The FAD synthetase from Corynebacterium ammoniagenes (CaFADS) is a bifunctional enzyme responsible for the synthesis of flavin mononucleotide (FMN) and flavin adenine dinucleotide (FAD) cofactors. The C-terminal module catalyzes FMN synthesis from riboflavin (RF) (riboflavin kinase, RFK), while the N-terminal one transforms FMN into FAD (FMN:adenylyltransferase, FMNAT). Bioinformatic tools for the exploration of macromolecular interfaces predict that CaFADS might stabilize in hexameric assemblies in solution, organized as dimer of trimers. In the predicted CaFADS dimer of trimers model, the protomers adopt a head-to-tail organization within each trimer that causes the RFK and FMNAT catalytic sites of two neighboring protomers 6 to be in proximity.

The overall structures of F206W, D298E and E301A CaFADSs are quite similar to that of the WT (A chains r.m.s.d. values 0.149, 0.152 and 0.251 Å, superimposing 274, 309 and 317 atoms, respectively). The E301A structure shows all residues in chain A but lacks 260, 261 and 262 in chain B. All mutant structures contain, in addition, one sulfate ion and one pyrophosphate molecule, as ligands in each chain. Finally, no conformational changes were observed in L6c or in the α1c helix, which contains the E301A mutation, when comparing this mutant’s structure to that of the WT. However, the H-bond between E301 of one protomer and T127 on loop L8n of the neighboring protomer, which is predicted for the WT dimer of trimers, is not expected in this case. E301 and L304 are predicted to interact with T127 and A132, respectively, of L8n of the neighboring protomer FMNAT site. The lack of interactions between the side chain of residue 301 and T127 in the E301A mutant and the substitution of L304 by Ala would both affect the van der Waals contacts with L8n in the dimer of trimers, producing local effects at this loop that helps close the FMNAT substrate binding site. These mutations can also alter the positive end of the helix α1c dipole, which contributes to the stability of substrate phosphate groups and is located near the FMNAT substrate binding site.

>[2x]MDIWYGTAAVPKDLDNSAVTIGVFDGVHRGHQKLINATVEKAREVGAKAIMVTFDPHPVSVFLPRRAPLGITTLAERFALAESFGIDGVLVIDFTRELSGTSPEKYVEFLLEDTLHASHVVVGANFTFGENAAGTADSLRQICQSRLTVDVIDLLDDEGVRISSTTVREFLSEGDVARANWALGRHFYVTGPVVRGAGRGGKELGFPTANQYFHDTVALPADGVYAGWLTILPTEAPVSGNMEPEVAYAAAISVGTNPTFGDEQRSVESFVLDRDADLYGHDVKVEFVDHVRAMEKFDSVAQLLEVMAKDVQKTRTLLAQDVQAHKMAPETYFLQAES> 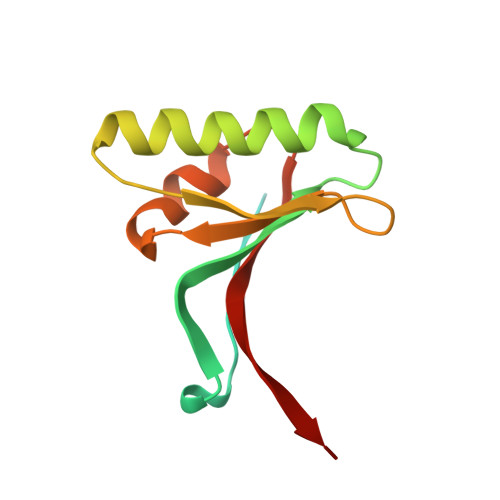QEDEDGDYEELVLALRSEEDGLAEAPEHGTTATFHRCAKDPWRLPGTYVVVLKEETHLSQSERTARRLQAQAARRGYLTKILHVFHGLLPGFLVKMSGDLLELALKLPHVDYIEEDSSVFAQ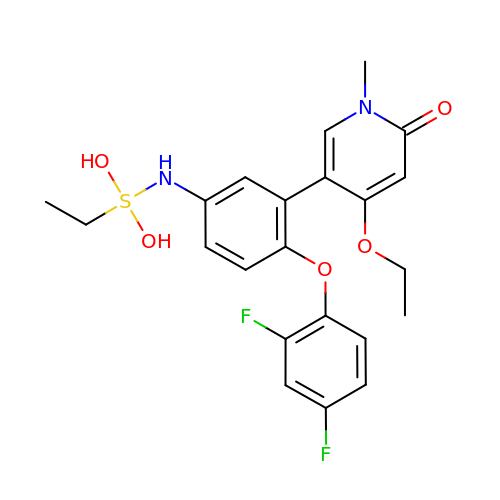5-[2-(2,4-difluorophenoxy)-5-{[ethyl(dihydroxy)-lambda~4~-sulfanyl]amino}phenyl]-4-ethoxy-1-methylpyridin-2(1H)-one | C22 H24 F2 N2 O5 S | JZIKIYOQVHKWKM-UHFFFAOYSA-N>[2x]RPEKPVYLSVKADNSMFIGNDPVTDETMITALNALTEGKKDTTIFFRADKTVDYETLMKVMDTLHQAGYLKIGLVGEETAKAK;> QPISVTMVTP

Gram-negative bacteria use TonB-dependent transport to take up nutrients from the external environment, employing the Ton complex to import a variety of nutrients that are either scarce or too large to cross the outer membrane unaided. The Ton complex contains an inner-membrane motor (ExbBD) that generates force, as well as nutrient-specific transport proteins on the outer membrane. These two components are coupled by TonB, which transmits the force from the inner to the outer membrane. Here, we identify a conserved motif within TonB that we term the D-box, which serves as an attachment point for ExbD.

The ExbD periplasmic domain alone yielded no crystals, even when high concentrations of protein were used (data not shown); however, crystals were readily obtained when the periplasmic domain was mixed with the D-box peptide. Two different crystal forms were obtained, both diffracting to approximately 1.4 Å; in each, the asymmetric unit comprises a 2:1 ExbD:D-box complex. Essentially identical structures are seen for the complex in two different crystal forms; in addition, these structures are highly similar to one recently published, which describes a 2:1 complex of the ExbD periplasmic domain with a 23-mer TonB peptide that includes the D-box sequence. Each ExbD monomer contains a five-stranded sheet, with two helices packed against one face of that sheet; two ExbD monomers assemble into a dimer with approximate two-fold symmetry. The two protomers contact one another via the loops connecting strand three and helix 2, imparting a V-shape to the dimer, with a deep groove between the two halves. The D-box peptide binds within this groove and, as hypothesized, assumes an extended conformation, forming a strand that is recruited to the edges of the beta sheets of both ExbD monomers. Thus, a single D-box strand is simultaneously recruited to the edges of two different beta sheets, one from each of the ExbD protomers. Because the D-box peptide adopts an extended conformation, the side chains of alternating residues point either up (toward solvent) or down (into the interface with ExbD). In particular, the side chains of Ile-57, Val-59, and Met-61 all point downward and are captured within hydrophobic cavities formed in the cleft between the two ExbD protomers. Met-61 lies at the C-terminal end of the D-box, and the hydrophobic pocket containing its side chain is partially formed by the side chain of Leu-132, offering an explanation for why the L132Q mutant fails to bind the D-box.> MRITTKVGDKGSTRLFGGEEVWKDSPIIEANGTLDELTSFIGEAKHYVDEEMKGILEEIQNDIYKIMGEIGSKGKIEGISEERIAW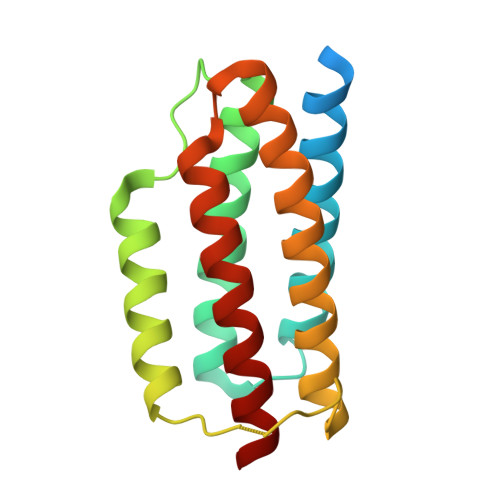LLKLILRYMEMVNLKSFVLPGGTLESAKLDVCRTIARRALRKVLTVTREFGIGAEAAAYLLALSDLLFLLARVIEIE>RDHRKIGKQLDLYHMQEEAPGMVFWHNDGWTIFRELEVFVRSKLKEYQYQEVKGPFMMDRVLWEKTGHWDNYKDAMFTTSSENREYCIKPMNCPGHVQIFNQGLKSYRDLPLRMAEFGSCHRNEPSGSLHGLMRVRGFTQDDAHIFCTEEQIRDEVNGCIRLVYDMYSTFGFEKIVVKLSTRPEKRIGSDEMWDRAEADLAVALEENNIPFEYQLGEGAFYGPKIEFTLYDCLDRAWQCGTVQLDFSLPSRLSASYVGEDNERKVPVMIHRAILGSMERFIGILTEEFAGFFPTWLAPVQVVIMNITDSQ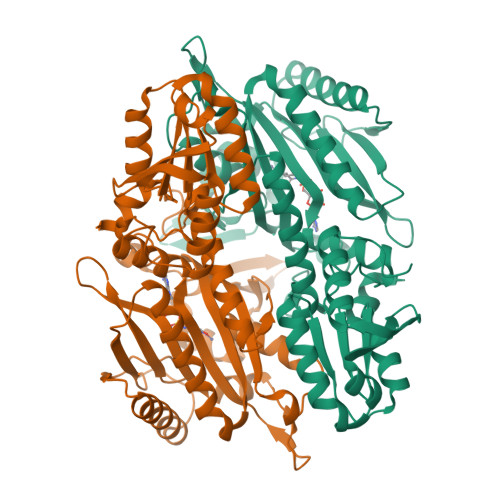SEYVNELTQKLSNAGIRVKADLRNEKIGFKIREHTLRRVPYMLVCGDKEVESGKVAVRTRRGKDLGSMDVNEVIEKLQQEIRSRSLKQLEE[4x]> MGTTLDDTAYRYRTSVPGDAEAIEALDGSFTTDTVFRVTATGDGFTLREVPVDPPLTKVFPDDESDDESDDGEDGDPDSRTFVAYGDDGDLAGFVVVSYSGWNRRLTVEDIEVAPEHRGHGVGRALMGLATEFARERGAGHLWLEVTNVNAPAIHAYRRMGFTLCGLDTALYDGTASDGEQ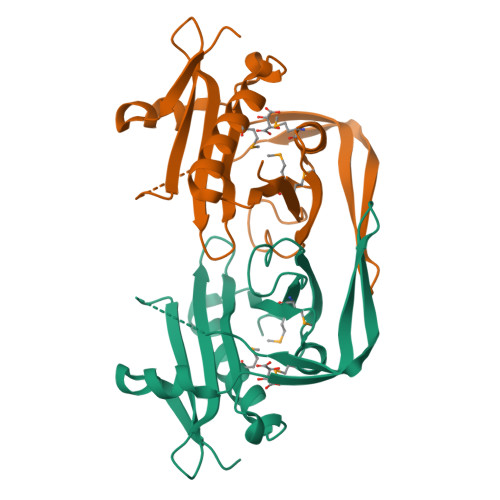ALYMSMPCP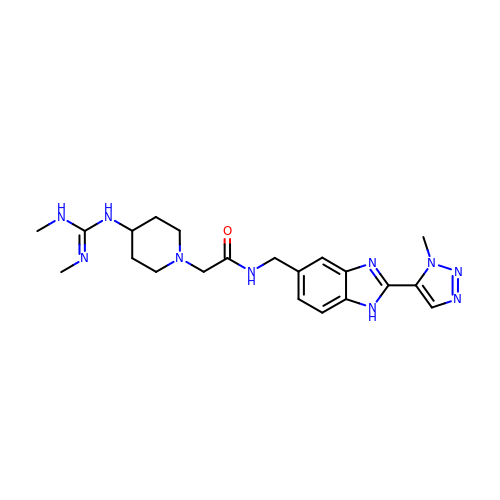2-[4-[[(~{E})-~{N},~{N}'-dimethylcarbamimidoyl]amino]piperidin-1-yl]-~{N}-[[2-(3-methyl-1,2,3-triazol-4-yl)-1~{H}-benzimidazol-5-yl]methyl]ethanamide | C21 H30 N10 O | XYBFHCJJYZWQNI-UHFFFAOYSA-N The 13 phospholipase C (PLC) isozymes expressed in humans preferentially hydrolyze the membrane phospholipid phosphatidylinositol 4,5-bisphosphate (PIP2) to generate the second messengers diacylglycerol and inositol 1,4,5-trisphosphate (IP3). The two PLC-γ isozymes, PLC-γ1 and PLC-γ2, are unique among the PLCs in that they are directly activated by tyrosine phosphorylation. PLC-γ1 and PLC-γ2 are phosphorylated on equivalent sites, Tyr783 and Tyr759, respectively, and this phosphorylation is typically required to stimulate phospholipase activity.

The 2.5 Å crystal structure of essentially full-length rat PLC-γ1 readily explains the autoinhibition of the PLC-γ isozymes. In addition, an internal loop of 25 residues connecting the cSH2 and SH3 domains was removed and replaced with a flexible linker; we refer to this internal deletion as Δ25. The crystallized construct therefore contains residues 21–765 and 791–1215 of PLC-γ1. In particular, the regulatory array sits ‘atop’ the conserved catalytic core and blocks the core from productively engaging membranes. However, in the case of PLC-γ1, the hydrophobic ridge interacts with portions of the sPH domain in the regulatory array; this arrangement is expected to effectively block membrane engagement. The active site sits beneath the hydrophobic ridge and is readily located by the bound Ca2+ cofactor. A second interface is formed between loops of the cSH2 domain and the C2 domain of the catalytic core. In this case, the BG and EF loops of the cSH2 domain clasp prominent turns of the C2 domain—almost as if the loops are pinching the C2 domain. The two interfaces between the regulatory array and catalytic core do not overlap, but the sPH and cSH2 domains within the regulatory array brace each other through the C-terminal portion of the SH3 domain that lies between them: picture an arch with the tail end of the SH3 domain acting as the keystone.

> SQAEVLHLCRSLEVGTVMTLFYSKKSQRPERKTFQVKLETRQITWSRGADKIEGSIDIREIKEIRPGKTSRDFDRYQEDPAFRPDQSHCFVILYGMEFRLKTLSLQATSEDEVNMWIKGLTWLMEDTLQAATPLQIERWLRKQFYSVDRNREDRISAKDLKNMLSQVNYRVPNMRFLRERLTDLEQRSGDITYGQFAQLYRSLMYSAQKTMDLPFLETNTLRTGERPELCQVSLSEFQQFLLEYQGELWAVDRLQVQEFMLSFLRDPLREIEEPYFFLDELVTFLFSKENSVWNSQLDAVCPETMNNPLSHYWISSSHNTYLTGDQFSSESSLEAYARCLRMGCRCIELDCWDGPDGMPVIYHGHTLTTKIKFSDVLHTIKEHAFVASEYPVILSIEDHCSIAQQRNMAQHFRKVLGDTLLTKPVDIAADGLPSPNQLKRKILIKHKKLAEGSAYEEVPTSVMYSENDISNSIKNGILYLEDPVNHEWYPHYFVLTSSKIYYSEETSSDQGNEDEEEPKEASGSTELHSSEKWFHGKLGAGRDGRHIAERLLTEYCIETGAPDGSFLVRESETFVGDYTLSFWRNGKVQHCRIHSRQDAGTPKFFLTDNLVFDSLYDLITHYQQVPLRCNEFEMRLSEPVPQTNAHESKEWYHASLTRAQAEHMLMRVPRDGAFLVRKRNEPNSYAISFRAEGKIKHCRVQQEGQTVMLGNSEFDSLVDLISYYEKHPLYRKMKLRYPINEEALEKIGSGSTFKCAVKALFDYKAQREDELTFTKSAIIQNVEKQDGGWWRGDYGGKKQLWFPSNYVEEMINPAILEPEREHLDENSPLGDLLRGVLDVPACQIAIRPEGKNNRLFVFSISMPSVAQWSLDVAADSQEELQDWVKKIREVAQTADARLTEGKMMERRKKIALELSELVVYCRPVPFDEEKIGTERACYRDMSSFPETKAEKYVNKAKGKKFLQYNRLQLSRIYPKGQRLDSSNYDPLPMWICGSQLVALNFQTPDKPMQMNQALFMAGGHCGYVLQPSTMRDEAFDPFDKSSLRGLEPCVICIEVLGARHLPKNGRGIVCPFVEIEVAGAEYDSTKQKTEFVVDNGLNPVWPAKPFHFQISNPEFAFLRFVVYEEDMFSDQNFLAQATFPVKGLKTGYRAVPLKNNYSEDLELASLLIKIDIFPAK> IGMAPGGYVAPKAVWLPAVKAK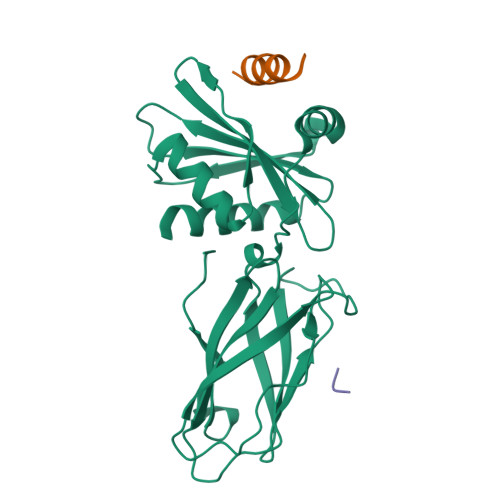GLEISGTFTHRQGHIYMEMNFTNKALQHMTDFAIQFNKNSFGVIPSTPLAIHTPLMPNQSIDVSLPLNTLGPVMKMEPLNNLQVAVKNNIDVFYFSCLIPLNVLFVEDGKMERQVFLATWKDIPNENELQFQIKECHLNADTVSSKLQNNNVYTIAKRNVEGQDMLYQSLKLTNGIWILAELRIQPGNPNYTLSLKCRAPEVSQYIYQVYDSILKN;>[2x]DDDIVFEDFARQRLKGMKDD> MGHHHHHHHHHHSSGHIEGRHMLRERTVRLQYGSRVEAVYVLGTYLWTDVYSAAPAGAQTFSLKHSEHVWVEVVRDGEAEEVATNGKQRWLLSPSTTLRVTMSQASTEASSDKVTVNYYDEEGSIPIDQAGLFLTAIEISLDVDADRDGVVEKNNPKKASWTWGPEGQGAILLVNCDRETPWLPKEDCRAEKVYSKEDLKDMSQMILRTKGPDRLPAGYEIVLYISMSDSDKVGVFYVENPFFGQRYIHILGRRKLYHVVKYTGGSAELLFFVEGLCFPDEGFSGLVSIHVSLLEYMAQDIPLTPIFTDTVIFRIAPWIMTPNILPPVSVFVCCMKDNYLFLKEVKNLVEKTNCELKVCFQYLNRGDRWIQDEIEFGYIEAPHKGFPVVLDSPRDGNLKDFPVKELLGPDFGYVTREPLFESVTSLDSFGNLEVSPPVTVNGKTYPLGRILIGSSFPLSGGRRMTKVVRDFLKAQQVQAPVELYSDWLTVGHVDEFMSFVPIPGTKKFLLLMASTSACYKLFREKQKDGHGEAIMFKGLGGMSSKRITINKILSNESLVQENLYFQRCLDWNRDILKKELGLTEQDIIDLPALFKMDEDHRARAFFPNMVNMIVLDKDLGIPK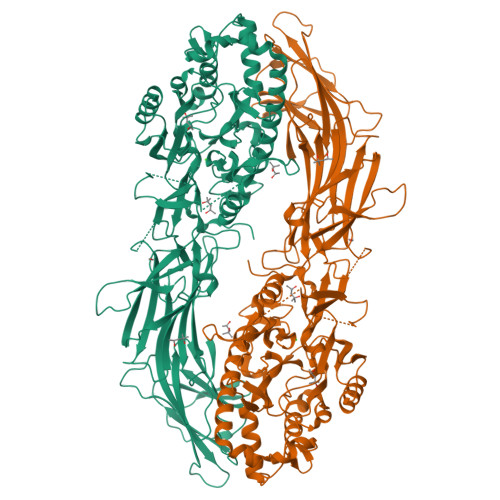PFGPQVEEECCLEMHVRGLLEPLGLECTFIDDISAYHKFLGEVHCGTNVRRKPFTFKWWHMVPSRRS>[3x]GSHMGQELVSLEGHQSAITALAFSKNIVVSGAADGTIKVWDILTGQLLRDHDGHQSEVTALQFKDNIVVSGAKDGTVKVWYIGTGQELVSLEGHQSAITALAFSKNIVVSGAADGTIKVWDILTGQLLRDHDGHQ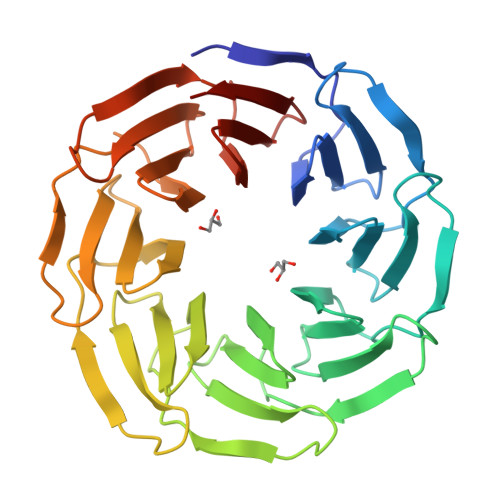SEVTALQFKDNIVVSGAKDGTVKVWYIGTGQELVSLEGHQSAITALAFSKNIVVSGAADGTIKVWDILTGQLLRDHDGHQSEVTALQFKDNIVVSGAKDGTVKVWYIGTGQELVSLEGHQSAITALAFSKNIVVSGAADGTIKVWDILTGQLLRDHDGHQSEVTALQFKDNIVVSGAKDGTVKVWYIGT> MSENKAPGQIYAYDIHNTHYPYVNIKQDSQTQLLASFRRSIASINPFSYRQVPSQDRAAFGLRWGNAWYAPNPYPNGIHFDRVFPTHYDPLAETNRTKANLQLIKYAPGNYSTLVVTSEKLPRPCIRTIQNYRRCQMVNGTEKCNSEAQDILAICPNWALDHMKEKVRFYTKALAINNQTYIRAMQVEEYNQGRTVADVAPKTWIHGTRQHLRPDTMWAD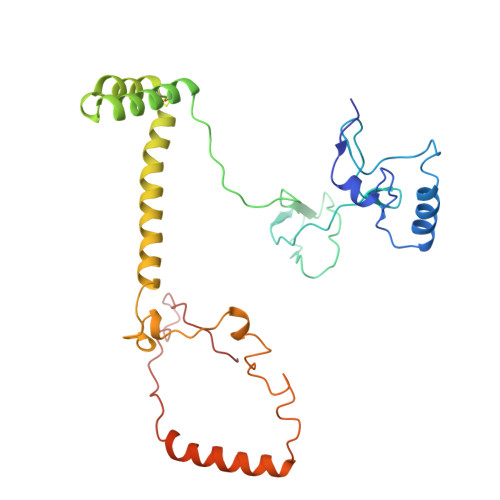DRYTNITQTEINEAIKRVEARKAREHEKKPVEQANVNANTGEQPVRVEKSLYP>[2x]ETPPRFTRTPVDQTGVSGGVASFICQATGDPRPKIVWNKKGKKVSNQRFEVIEFDDGSGSVLRIQPLRTPRDEAIYECVASNNVGEISVSTRLTVLREDQIPRGFPTIDMGPQLKVVERTRTATMLCAASGNPDPEITWFKDFLPVDTSN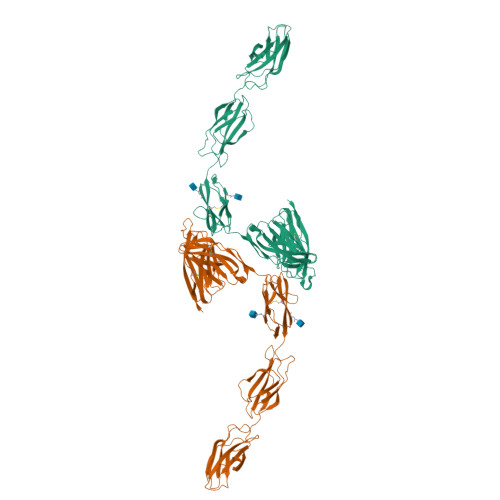NNGRIKQLRSESIGALQIEQSEESDQGKYECVATNSAGTRYSAPANLYVRVRRVPPRFSIPPTNHEIMPGGSVNITCVAVGSPMPYVKWMLGAEDLTPEDDMPIGRNVLELNDVRQSANYTCVAMSTLGVIEAIAQITVKALPKPPGTPVVTESTATSITLTWDSGNPEPVSYYIIQHKPKNSEEPYKEIDGIATTRYSVAGLSPYSDYEFRVVAVNNIGRGPASEPVLTQTSEQAPSSAPRDVQARMLSSTTILVQWKEPEEPNGQIQGYRVYYTMDPTQHVNNWMKHNVADSQITTIGNLVPQKTYSVKVLAFTSIGDGPLSSDIQVITKHHHHHH(1~{R},2~{S})-2-[[4-[[3-(aminomethyl)phenyl]amino]quinazolin-2-yl]amino]cyclohexane-1-carboxylic 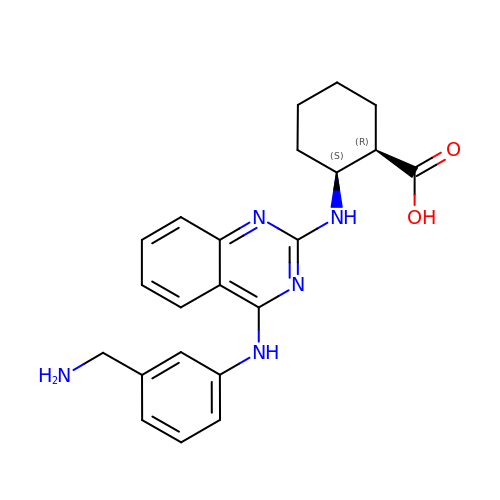acid | C22 H25 N5 O2 | HGCXJWRMCKMKEG-MJGOQNOKSA-N>[5x]MAVSTVTGAAGIGLATLAADGSVLDTWFPAPELTESGTSATSRLAVSDVPVELAALIGRDDDRRTETIAVRTVIGSLDDVAADPYDAYLRLHLLSHRLVAPHGLNAGGLFGVLTNVVWTNHGPCAIDGFEAVRA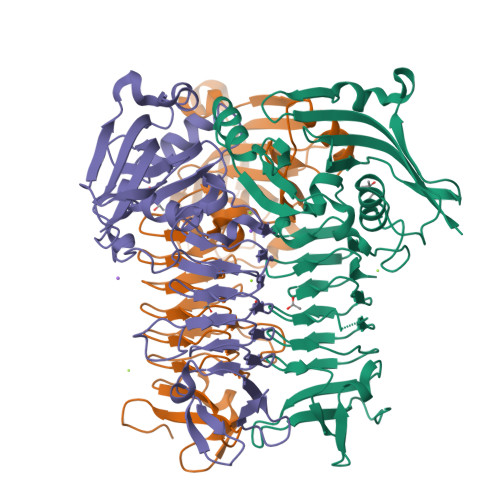RLRRRGPVTVYGVDKFPRMVDYVVPTGVRIADADRVRLGAHLAPGTTVMHEGFVNYNAGTLGASMVEGRISAGVVVGDGSDVGGGASIMGTLSGGGTHVISIGKRCLLGANSGLGISLGDDCVVEAGLYVTAGTRVTMPDSNSVKARELSGSSNLLFRRNSVSGAVEVLARDGQGIALNEDLHANGVPRGLEHHHHHH>GPMEPRSMEYFCAQVQQKDVGGRLQVGQELLLYLGAPGAISDLEEDLGRLGKTVDALTGWVGSSNYRVSLMGLEILSAFVDRLSTRFKSYVAMVIVALIDRMGDAKDKVRDEAQTLILKLMDQVAPPMYIWEQLASGFKHKNFRSREGVCLCLIETLNIFGAQPLVISKLIPHLCILFGDSNSQVRDAAILAIVEIYRHVGEKVRMDLYKRGIPPARLEMIFAKFDEVQS[2x]

Cytoplasmic linker-associated proteins (CLASPs) are excellent candidates to promote MT growth because they are well known to increase MT abundance and stability in mitosis and interphase. CLASP1α and 2α consist of three TOG-like domains (termed TOG1, 2, and 3) and a C-terminal domain responsible for interactions with CLIP-170 and other partners, CLIP-interacting domain (CLIP-ID) (Akhmanova et al., 2001, Al-Bassam and Chang, 2011). Mammalian CLASPs encompass three TOG-like domains, TOG1, TOG2, and TOG3, none of which bind to free tubulin. CLASPs suppress catastrophes by stabilizing growing microtubule ends, including incomplete ones, preventing their depolymerization and promoting their recovery into complete tubes.

To understand why TOG1 does not bind to free tubulin, we solved its structure by X-ray crystallography. The structure of TOG1 showed a conserved TOG-domain fold, but also demonstrated that the conserved residues required for tubulin interaction are lacking. This explains why TOG1 does not bind to either free tubulin or MTs. We also checked whether TOG1 could bind to alternative tubulin structures, such as tubulin rings induced by dolastatin or vinblastine, but found this not to be the case. We confirmed that the binding of TOG2 and TOG3 to stabilized MTs was weak, while TOG1 and CLIP-ID did not bind to MTs at all, and none of these domains interacted with free tubulin. Strikingly, the deletion of this domain (which converted CLASP2α to the equivalent of the naturally occurring splice isoform CLASP2γ), strongly diminished the ability of CLASP2 to suppress catastrophes, in agreement with a previous publication (Yu et al., 2016). To explain these results, we hypothesized that CLIP-ID has an auto-inhibitory activity that can be relieved by TOG1. Addition of this construct potently increased the anti-catastrophe activity of all TOG2-containing CLASP2 constructs that lacked TOG1 but contained CLIP-ID. These results suggest that CLIP-ID, when it is not bound to partners such as CLIP-170, has an inhibitory effect on TOG2, and possibly also on TOG3, while TOG1 can relieve this inhibition. Thus, in contrast to a previous publication suggesting that the ability of TOG1 to bind free tubulin is required for CLASP activity (Yu et al., 2016), we establish that TOG1 has an autoregulatory function. TOG1 is present in CLASP1/2α but absent in CLASP2β and CLASP2γ isoforms (Akhmanova et al., 2001).>AQPIVIKFSHVVAENTPKGQGALLFKKLVEQRLGGRVEVDVYPNSSLFGDGKEMEALLLGDVQMLAPSLAKFEQYTRKVQIFDLPFLFDDIQAVDRFQRSPQGRALLTSMQGKGILGLAYWHNGMKQLSANRPLLEPEDARGLKFRVQASDVLNEQFRQLRAISRKMSFAEVYQGLQTGVVNGTENTWSNYESQKVNEVQKYFTESNHGLVDYMVITNAKFWNGLPADIREELQRIMDEVTVQVNLEAERLNRDARQRILASGASEIHTLSPQQRADWRQAMQPVWQKFRGNVGADLLQAAEASNRPD[2x]

Here, we demonstrate that a genetically linked tripartite ATP-independent periplasmic (TRAP) transporter (pa0884-pa0886), which is homologous to the known C4-dicarboxylate-binding TRAP system, is essential for growth on itaconate, but not for the closely related C4-dicarboxylate succinate. Using tryptophan fluorescence spectroscopy, we demonstrate that the substrate-binding protein (SBP), IctP (PA0884), binds itaconate but still retains higher affinity for the related C4-dicarboxylates. The structures of IctP bound to itaconate (1.80 Å) and succinate (1.75 Å) revealed an enclosed ligand-binding pocket with ion pairing interactions with the ligand carboxylates. The C2 methylene group that is the distinguishing feature of itaconate compared with succinate is accommodated by a unique change in the IctP-binding site from a Leu to Val, which distinguishes it from closely related C4-dicarboxylate-binding SBPs. Together, these data suggest that this transporter, which we name IctPQM, has duplicated from a canonical C4-dicarboxylate transporter, and its evolution towards itaconate specificity enables this pathogen to now access a key metabolite for persistence in the host.

The proximal (C1) carboxylate group forms a two-pronged ion-pair with the guanidino moiety of R169, a key characteristic of a DctP family SBP ligand interaction, further interacting with the ε-amino group of K94, the amide –NH2 of N209 and an ordered water molecule. Meanwhile, the distal (C4) carboxylate forms polar interactions with the charged amino group of the K41 side chain, the amide –NH2 moiety of the side chain of N213, the phenolic hydroxyl of Y236 and a further ordered water molecule. These polar interactions are supplemented by apolar interactions involving the side chains of V34, V35, S91, F192 and V234. The nearest neighbours of the methylene substituent are provided by the side chains of Q171, V234 and S91. This group is otherwise enclosed by the K94 side chain and a water molecule. The alteration from the larger leucine residue in DctP to the smaller valine in IctP suggests that V234 could be the primary adaptation in IctP that enables it to recognise itaconate with μM affinity. In an identical binding site, the larger L234 residue found in DctP would likely interfere with the accommodation of itaconate in the binding.>GHMPSAQIIDGKAIAAAIRSELKDKVAALRELYGGRVPGLASIIVGQRMDSKKYVQLKHKAAAEVGMASFNVELPEDISQEVLEVNVEKLNNDPNCHGIIVQLPLPKHLNENRAIEKIHPHKDADALLPVNVGLLHYKGREPPFTPCTAKGVIVLLKRCGIEMAGKRAVVLGRSNIVGAPVAALLMK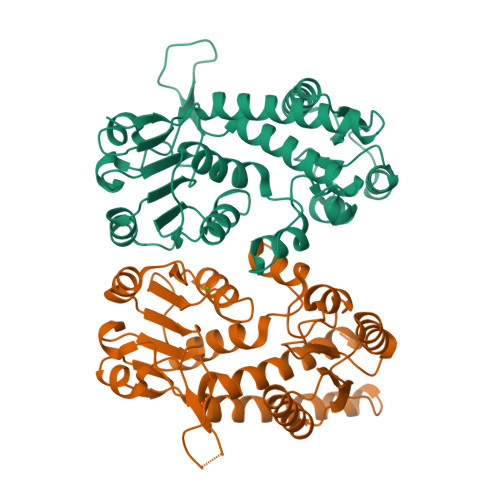ENATVTIVHSGTSTEDMIDYLRTADIVIAAMGQPGYVKGEWIKEGAAVVDVGTTPVPDPSRKDGYRLVGDVCFEEAAARAAWISPVPGGVGPMTIAMLLENTLEAFKAALGVS[2x]>[2x]ADSDVPNDILEEQLYNSVVVADYDSAVEKSKHLYEEKKSEVITNVV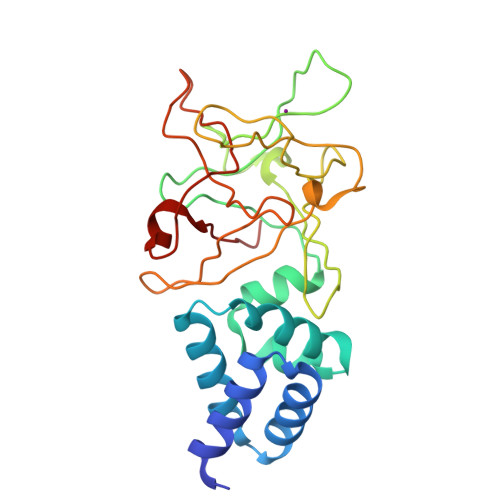NKLIRNNKMNCMEYAYQLWLQGSKDIVRDCFPVEFRLIFAENAIKLMYKRDGLALTLSNDVQGDDGRPAYGDGKDKTSPRVSWKLIALWENNKVYFKILNTERNQYLVLGVGTNWNGDHMAFGVNSVDSFRAQWYLQPAKYDNDVLFYIYNREYSKALTLSRTVEPSGHRMAWGYNGRVIGSPEHYAWGIKAF> MESLPVIAAPSMWTRPQIKDFKEKIQQDADSVITVGRGEVVTVRVPTHEEGSYLFWEFATDNYDIGFGVYFEWTDSPNTAVSVHVSESSDDDEEEEENIGCEEKAKKNANKPL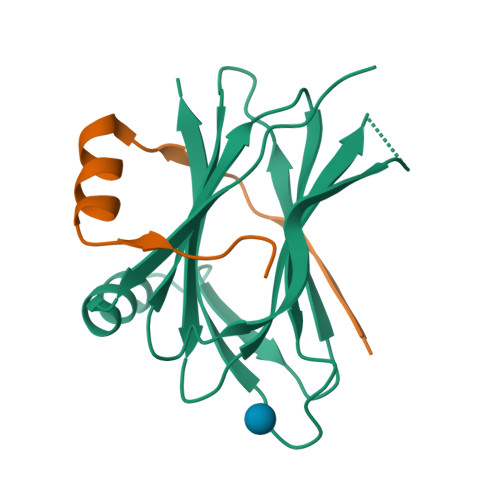LDEIVPVYRRDCHEEVYAGSHQYPGRGVYLLKFDNSYSLWRSKSVYYRVYYTR;> GAHSERTFETAPSEIDADEVLEILSKSKPAPTHLTLER8-(benzyloxy)-5-chloroquinoline | C16 H12 Cl 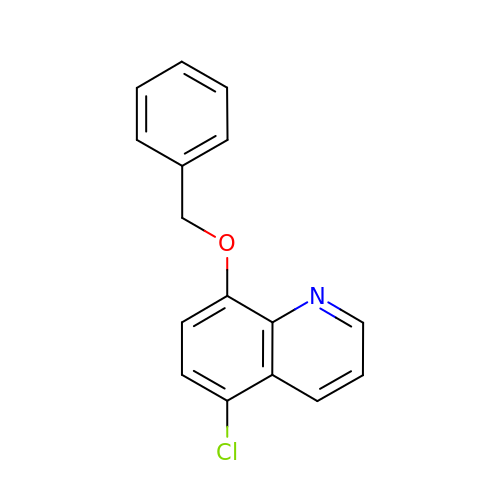N O | LPPVIXWNCVGAJV-UHFFFAOYSA-N> DERSWVYSPLHYS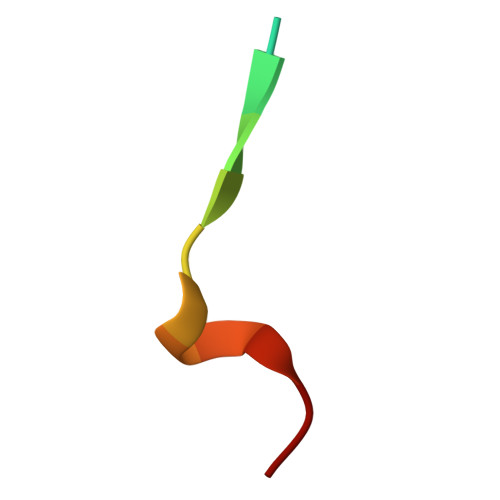A>[4x]GSMENLLEEVEKAKVIADEAVK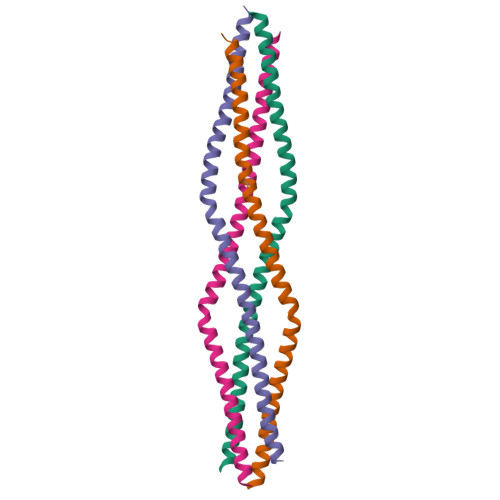LQKEIDKRCQHKIAEMVALMEKHKHQYDKIIEERDSELGLYKSKEQEQSSLRASLEIELSNLKAELLSVKKQLEIE> LGSPGIQGEVVDCHLSDMLQQLHSVNASKPSERGLVRQEEAEDPACIPIFWVSKW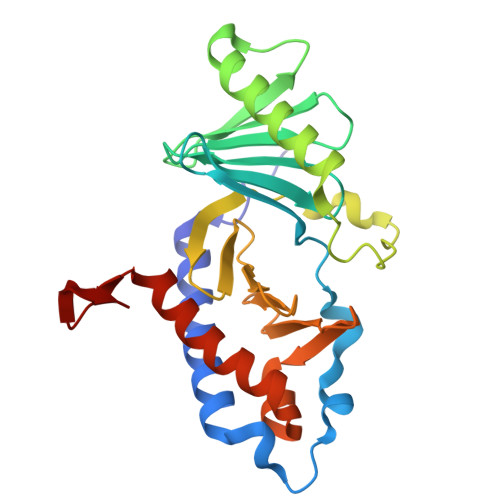VDYSDKYGLGYQLCDNSVGVLFNDSTRLILYNDGDSLQYIERDGTESYLTVSSHPNSLMKKITLLKYFRNYMSEHLLKAGANITPREGDELARLPYLRTWFRTRSAIILHLSNGSVQINFFQDHTKLILCPLMAAVTYIDEKRDFRTYRLSLLEEYGCCKELASRLRYARTMVDKLLSSRSASNRLKAS>CGCGC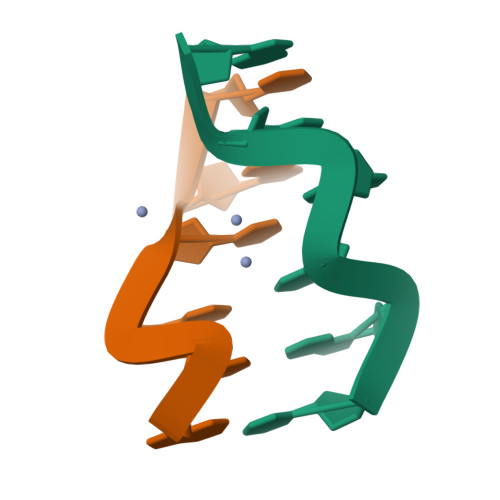G[2x]>MESAIDTHLKCPRTLSRRVPEEYQPPFPMWVARADEQLQQVVMGYLGVQYRGEAQREAALQAMRHIVSSFSLPDGPQTHDLTHHTDSSGFDNLMVVGYWKDPAAHCRWLRSAEVNDWWTSQDRLGEGLGYFREISAPRAEQFETLYAFQDNLPGVGAVMDSTSGEIEEHGYWGSMRDRFPISQTDWMKPTNELQVVAGDPAKGGRVVIMGHDNIALIRSGQDWADAEAEERSLYLDEILPTLQDGMDFLRDNGQPLGCYSNRFVRNIDLDGNFLDVSYNIG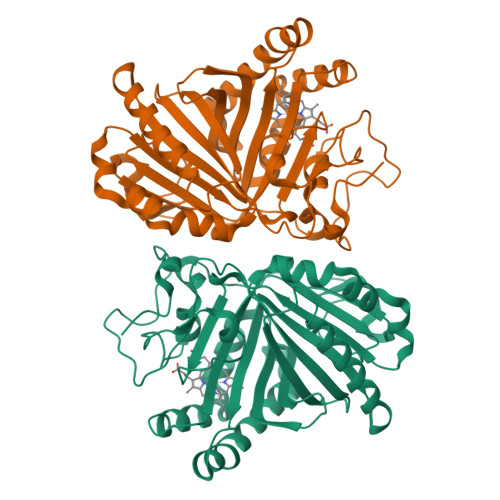HWRSLEKLERWAESHPTHLRIFVTFFRVAAGLKKLRLYHEVSVSDAKSQVFEYINCHPHTGMLRDAVVAPT[2x]>[2x]RASQQIPWGIKAIYNNDTLTSTTGGSGINIAVLDTGVNTSHPDLVNNVEQCKDFTGATTPINNSCTDRNGHGTHVAGTALADGGSDQAGIYGVAPDADLWAYKVLLDSGSGYSDDIAAA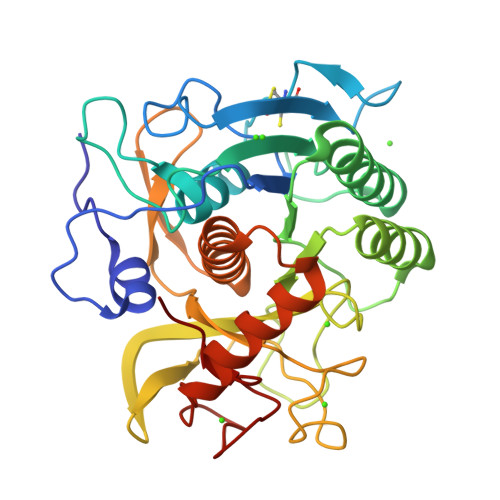IRHAADQATATGTKTIISMSLGSSANNSLISSAVNYAYSKGVLIVAAAGNSGYSQGTIGYPGALPNAIAVAALENVQQNGTYRVADYSSRGYISTAGDYVIQEGDIEISAPGSSVYSTWYNGGYNTISGTSMATPHVSGLAAKIWAENPSLSNTQLRSNLQERAKSVDIKGGYGAAIGDDYASGFGFARVQ Here, we demonstrate that MavC actually targets the Ube2N–Ub conjugate to catalyze an intramolecular transglutamination reaction. MavC-catalyzed transglutamination proceeds via an obligate thioester-linked intermediate to form an isopeptide bond between Gln40Ub and Lys92Ube2N. Architecturally, MavC1–384 is composed of three distinct lobes: a core globular domain (CG) flanked by an insertion domain (residues 128–225) on one end and an α-helical extension (HE: residues 33–66, 356–384) on its opposite end. Ubiquitination of Lys92Ube2N, located adjacent to the E2 active site, effectively inhibits Ube2N activity and attenuates downstream host NF-κB activation.

The MavC insertion domain can be expressed and purified on its own, and a crystal structure of the insertion domain shows that it preserves an identical fold to that in the full MavC protein. BLI and glutathione-s-transferase (GST) pulldown experiments show that the isolated insertion domain is able to bind to Ube2N independently and with an affinity comparable to full-length MavC. An analogous NMR titration using purified MavC insertion domain (MavC128–225) yielded Ube2N spectral changes that are remarkably similar to those observed with C74A-MavC1–384 despite the large molecular weight differences. These observations suggest that the MavC insertion domain is primarily responsible for binding Ube2N, a conclusion supported by similar Kd values obtained from BLI measurements of Ube2N binding to MavC or the MavC insertion domain. The insertion domain appears to behave as an independent Ube2N-binding domain but when built into MavC its rotational states provide specific functionality during the transamidation reaction.

>GPLGSRFNAPQKYQKIKREEFNPETAEKNKIYLLEDQLVYLDIFGKVIDLGQTSDTCHRLFNAITTPFYQNYILYDEYIDPEESAEEAAMFEMGEIVKAKMKNID[2x]> MVHHHHHHLLVPRGSKIEEVKSTTKTQRIASHSHVKGLGLDESGLAKQAASGLVGQENAREACGVIVELIKSKKMAGRAVLLAGPPGTGKTALALAIAQELGSKVPFCPMVGSEVYSTEIKKTEVLMENFRRAIGLRIKEGPPGIIQDVTLHDLDVANARPQGGQDILSMMGQLMKPKKTEITDKLRGEINKVVNKYIDQGIAELVPGVLFVDEVHMLDIECFTYLHRALESSIAPIVIFASNRGNCVIRGTEDITSPHGIPLDLLDRVMIIRTMLYTPQEMKQIIKIRAQTEGINISEEALNHLGEIGTKTTLRYSVQ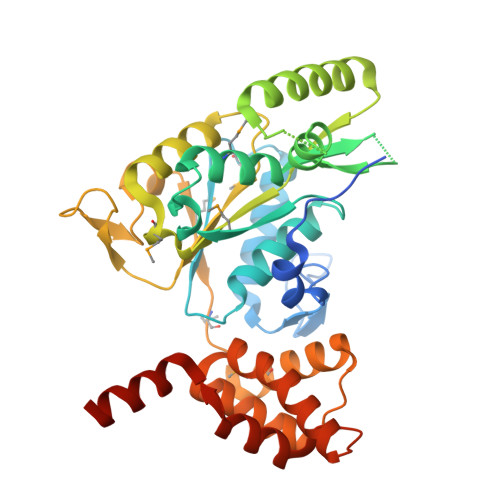LLTPANLLAKINGKDSIEKEHVEEISELFYDAKSSAKILADQQDKYMK>NAQFLHTQVGRGLLGAVVNPLGEVTDKFAVTDNSEILYRPVDNAPPLYSERAAIEKPFLTGIKVIDSLLTCGEGQRMGIFASAGCGKTFLMNMLIEHSGADIYVIGLIGERGR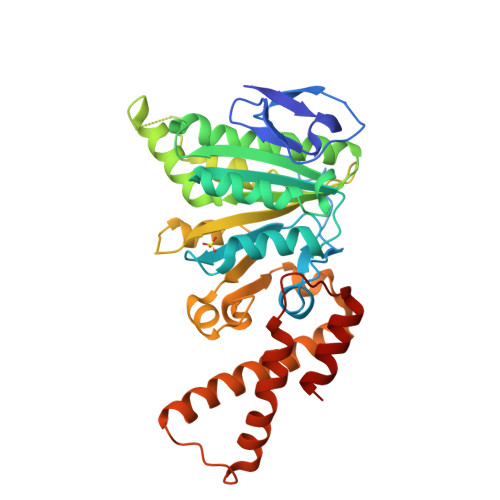EVTETVDYLKNSEKKSRCVLVYATSDYSSVDRCNAAYIATAIAEFFRTEGHKVALFIDSLTRYARALRDVALAAGESPARRGYPVSVFDSLPRLLERPGKLKAGGSITAFYTVLLEDDDFADPLAEEVRSILDGHIYLSRNLAQKGQFPAIDSLKSISRVFTQVVDEKHRIMAAAFRELLSEIEELRTIIDFGEYKPGENASQDKIYNKISVVESFLKQDYRLGFTYEQTMELIGETIR[2x]>[2x]MGHHHHHHSHMELYECIQDIFGGLKNPSVKDLATSLKQIPNAAKLSQPYIKEPDQYAY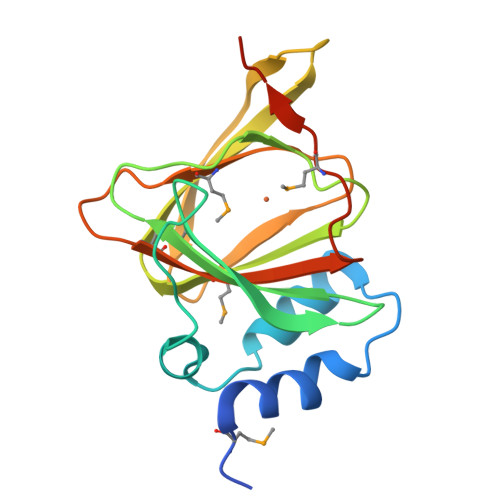GRNAIYRNNELEIIVINIPPNKETTVHDHGQSIGCAMVLEGKLLNSIYRSTGEHAELSNSYFVHEGECLISTKGLIHKMSNPTSERMVSLHVYSPPLEDMTVFEEQKEVLENS The 12-kDa FK506-binding protein (FKBP12) is a ubiquitously expressed peptidyl-prolyl isomerase with considerable homology between fungal pathogens and is thus a prime candidate for future targeting efforts to generate a panfungal strategy. PPIase proteins all catalyze the cis/trans isomerization of peptide bonds N terminal to proline residues in polypeptide chains. In addition to its role as a PPIase, FKBP12 is a member of the immunophilin family and is the target of the immunosuppressive drugs FK506 and rapamycin. Three extended loops, which have been called the 40s loop (between β2 and β3), the 50s loop (between β3′ and α1), and the 80s loop (between β4 and β5), surround a deep active-site pocket that binds both FK506 and rapamycin.

Thus, to assess if this interaction occurs in solution, we made a single cysteine mutation, V91C, in the A. fumigatus protein to try to capture a disulfide cross-linked complex. This residue was chosen for mutation because the structure revealed that the V91 and V91′ (where the prime indicates the other subunit of the dimer) side chains are within <4.0 Å of each other and that when they are mutated to cysteines in silico they could form a disulfide bond in the intermolecular dimer. When the proteins were purified from both strains in the absence of a reducing agent and subjected to nonreducing SDS-PAGE, the samples revealed the presence of two species, which were consistent with FKBP12 monomers and dimers. When a reducing agent (β-mercaptoethanol) was added, the proteins ran as monomers. We next separated the V91C dimer from the monomer via size exclusion chromatography and crystallized and solved the structure of the dimer to 3.2 Å resolution. The structure revealed a disulfide cross-linked dimer. Interestingly, although revealing the same general dimer that we observed in the A. fumigatus and C. albicans apo FKBP12 structures, in the FKBP12(V91C) structure, Pro90 is slightly shifted from the active site and adopts a twisted conformation, suggesting that the structure may have captured an intermediate state of catalysis. In fact, the conformation of the Pro90 residues in the structure is closer to the trans than the cis state and overlays of the trans state of the protein to form an all-trans dimer revealed a clash. This finding suggests the intriguing possibility that part of the mechanism of prolyl isomerization by FKBPs is dictated by the conformation of the substrate during catalysis.

>[2x]MGVTKELKSPGNGVDFPKKGDFVTIHYTGRLTDGSKFDSSVDRNEPFQTQIGTGRVIKGWDEGVPQMSLGEKAVLTITPDYGYGARGFPPCIPGNSTLIFEVELLGINNKR>[2x]ATALTNLVAEPFAKLEQDFGGSIGVYAMDTGSGATVSYRAEERFPLCGSFKGFLAAAVLARSQQQAGLLDTPIRYGKNALVPWSPISEKYLTTGMTVAELSAAAVQYSDNAAANLLLKELGGPAGLTAFMRSIGDTTFRLDRWELELNSAIPGDARDTSSPRAVTESLQKLTLGSALAAPQRQQFVDWLKGNPTGNHRIRAAVPADWAVGDKTGTCGVYGTA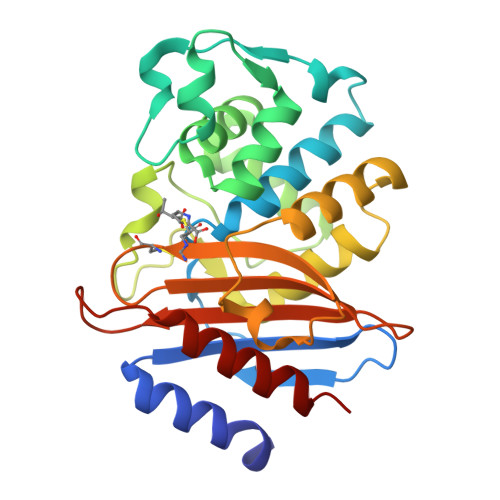NDYAVVWPTGRAPIVLAVYTRAPNKDDKHSEAVIAAAARLALEGLG>SGIRELNLTKEQHEWLNGWLELWGAWVYSGRLEKRMSSVIAKFMESVEPGRVMTRPMCNDDDGMLISQVVDSVMYIDKKAFGILLSYYAHGSSKHAIASYYHRVARPRKMLCRGGGRIQKPSLATCRREVDEILNASLFMIYPVLDSAFKN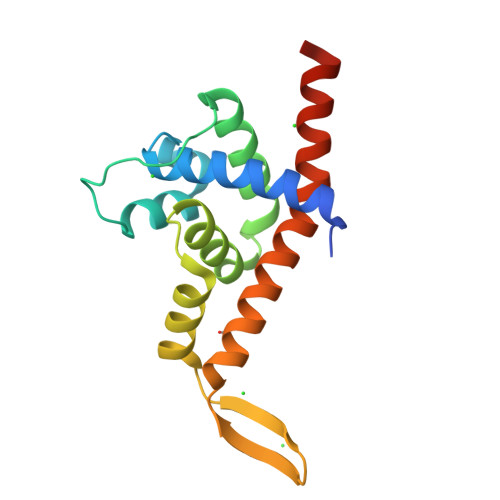RKRVEKIKHVA[2x]The polymerase-associated factor 1 complex (PAF1C) is one of the most important transcription elongation factors that positively regulates genome-wide gene expression. In simple eukaryotes such as budding yeast, PAF1C contains five subunits: Paf1, Ctr9, Cdc73, Leo1 and Rtf1. PAF1C can regulate transcription through direct association with the polymerase or by impacting the chromatin structure epigenetically. The largest component, Ctr9, forms the backbone and shapes the overall architecture of the complex, while the other components join the complex mainly through associations with Ctr9.

In this study, we solved a high-resolution quaternary PAF1C of Ctr9-Paf1-Cdc73-Rtf1 from Saccharomyces eubayanus. The major body of Ctr9 folds into 21 tetratricopeptide repeats (TPRs) that wrap around the N-terminus of Paf1 to form a three-circled right-handed solenoid structure, with the Paf1 N-terminus just filling in the central tunnel of the Ctr9 solenoid. The rest of Paf1 extends out from the central tunnel and contacts the outer surface of Ctr9. Cdc73 and Rtf1 contact mainly the outer surface of Ctr9. Their interactions with Ctr9 were further strengthened by inserting a fragment into the groove of Ctr9 and making contacts with residues within the groove. Cdc73 without the α1 helix still formed a complex with the Ctr9-Paf1-Rtf1 ternary complex, while Cdc73 without α2 could no longer join the ternary complex, indicating that the hydrophobic contacts by the C-terminal α2 are critical for Cdc73 to associate with Ctr9. Rtf1 contacts Ctr9 spanning a region including the lower part of the N-terminal turn and the upper part of the middle turn of Ctr9. As Rtf1 and Cdc73 occupy different regions of Ctr9, they do not have direct interactions within this core structure. Residues 531 to 552 of Rtf1 form the bottom of the letter “U” that lie in the groove of Ctr9. In contrast, Rtf1 without the C-terminal tail or with only the C-terminal tail showed reduced binding to the ternary complex, indicating that the very C-terminus and the segment that binds within the groove of Ctr9 are two key segments important for Rtf1 to associate with PAF1C.

> SGSAGNGLVPSDPVLAETMKNERVVQDHNSALRGARPINFGYLIKDAELKLVQSIKGSLRGSKLPPGHKGAHGRVSKTNGS;> MANTIKVEGYPSMEWPTSLDIPLKASEELVGIDLETDLPDDPTDLKTLLVEESSEKEHWLTIALAYCNHGKTNEGIRLIEMALDVFQNSERASLHTFLTWAHLNLAKGHSLSVETKEHELTQAELNLKDAIGFDPTWIGNMLATVELYYQRGHYDKALETSDLFVKSIHAEDHRSGRQSKPNCLFLLLRAKLLYQKKNYVASLKIFQELLVINPVLQPDPRIGIGLCFWQLKDPKMAIKSWQRALQINSKNTSASILVLLGEFHNSLTDSTNDEVFKETFSKALSDLKNIFSENQNNPVLLTLLQTYHYFKGDFQTVLDIYHHKILKMSPLIAKTVLSESSFWCGRAHYALGDYRKSFIMFQESLKKNEDNLMARLGLGQTQIKSNLLEESIITFENLYKTNESLQELNYILGLLYAGKTLDVKTSKSIPAKELNKLNEKALQYLERYIKLTVAKKNQLIISRVYLVISQLYESQNQYKISLDFLSKALEEMEFVNKDEVPLEILNNLACYHFINGDLTKADNLFEQAKAKVSDMNKSVNITLEYNIARTSEKTNWEKSESIYSQITSSHPSYISARIRNLYIKFAHSKINDSEMNIEINGLLEMNKSDLEMRSFYGWYLKNSEERKNSEKSTSHNKETLVKYNSHDAYALISLANLYVTIARDGKKSRNPKEQEKSKHSYLKAIQLYQKVLQIDPFNVFAAQGVAIIFAESKRLGPALEILRKIRDSLDNEDVQLNLAHCLLEMREFGKAIENYELVLKKFDNERTRPHILNLLGRAWYSRGMKERSVSFFQKALENAKTALELFVQQSAKNKFIHSVKFNIALLQFQIAETLRRSNPKFRTVQQIKDSLEGLEEGLALFKELNDLKEFNMIPKEELEQRIQLGETTMKSALERSLNEQEEFEKDQ;> SMSKKQEYIAPIKYQNSLPVPQLPPKLLAYPEAPETNPDSSQLINSLYVKTNISNLIQQDEDLGMPVDLMKFPGLLNKLDSKLLYGFDNVKLDKDDRILLRDPRIDRLTKT;> SKSDPFSRLKTRTKVYYQEIQKEENAKAKEMAQQEKLQEDRETKERREKELLLAQFRRLGGLERMIGELDIKFDFKF> NYSNEFGLMQPIQEFKAFIES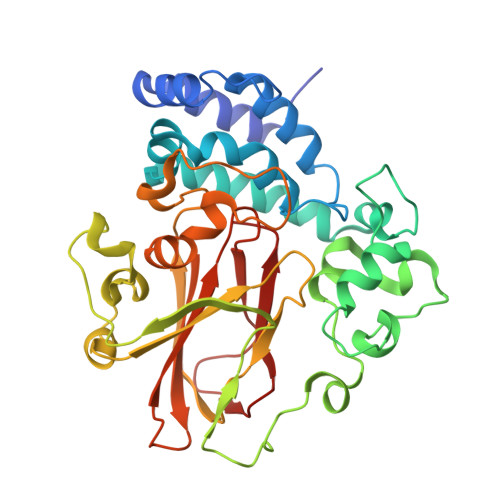DPVVHQEFIDMFEGIQDSPRNYQELCNMFNDIFRKAPVYGDLGPPVYMIMAKLMNTRAGFSAFTRQRLNLHFKKLFDTWGLFLSSKDSRNVLVADQFDDRHCGWLNERALSAMVKHYNGRAFDEVFLCDKNAPYYGFNSYDDFFNRRFRNRDIDRPVVGGVNNTTLISAACESLSYNVSYDVQSLDTLVFKGETYSLKHLLNNDPFTPQFEHGSILQGFLNVTAYHRWHAPVNGTIVKIINVPGTYFAQAPSTIGDPIPDNDYDPPPYLKSLVYFSNIAARQIMFIEADNKEIGLIFLVFIGMTEISTCEATVSEGQHVNRGDDLGMFHFGG>MGHHHHHHGGHMSLLRFLEVVSEHIKNLRNHIDLETVGEMIKLIDSARSIFVIGAGRSGYIAKAFAMRLMHLGYTVYVVGETVTPRITDQDVLVGISGSGETTSVVNISKKAKDIGSKLVAVTGKRDSSLAKMADVVMVVKGKMKQERDEILSQLAPLGTMFELTAMIFLDALVAEIMMQKHLT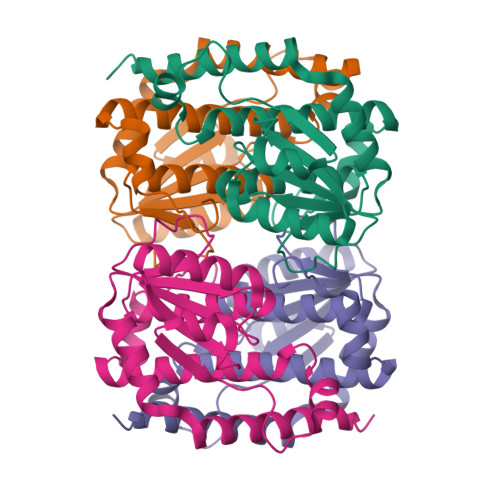EKDLEARHAVLEEGGS[4x]> MIASSPIDAAALRASVAAALDPSTAVATLARFDTHAPRLLDALSTLYGDHADYVTWLPQWLSALGVVAQARPAALRHLDDSRAPGWFGQQDMLGYSAYVDRFAGTLRGVAERVPYLQELGVRYLHLLPFLRARAGDNDGGFAVSDYGQVEPALGSNDDLVALTARLRAANISLCADFVLNHTADDHAWAQAARAGDTRYLDYYHHFADRNAPDQYDTTLVQVFPQTAPGNFTWVDETRQWMWTTFYPYQWDLNWSNPAVFGEMALAMLELANLGVEAFRLDSTAYLWKRPGTNCMNQPEAHTILVALRAVADIVAPSVVMKAEAIVPMAELPPYFGSGVQRGHECHLAYHSTLMAAGWSALALQRGDILQDVIAHSPPLPPNCAWLSYVRCHDDIGWNVLQHEAAGTAAQPPFSLREVAQFYANAVPGSYARGESFQSSGDGVHGTNGMSAALVGVQAAHEHADAAAAARAVDRLVLLYAVSLAMPGVPLIYMGDELALPNDTAYLDDAQRRHEGRWLHRPAMAWELAAQRHDASTLAGTVYTRLRALIRLRAGLPALAATQSLGSVALGDARLFALTR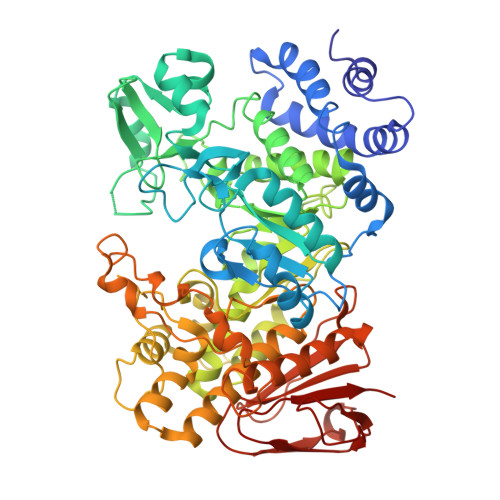GDSFLAVHNFSDVPLPVDLTQTGHALWAVLDTDGTGDAPEPHTELLLPAYGVRWLQRR> MENKTETTVRRRRRIILFPVPFQGAINPILQLANVLYSKGFSITIFHTNFNKPKTSNYPHFTFRFILDNDPQDERISNLPTHGPLAGMRIPIINEHGADELRRELELLMLASEEDEEVSCLITDALWYFAQSVADSLNLRRLVLMTSSLFNFHAHVSLPQFDELGYLDPDDKTRLEEQASGFPMLKVKDIKSAYSNWQILKEILGKMIKQTKASSGVIWNSFKELEESELETVIREIPAPSFLIPLPKHLTASSSSLLDHDRTVFQWLDQQPPSSVLYVSFGSTSEVDEKDFLEIARGLVDSKQSFLWVVRPGFVKGSTWVEPLPDGFLGERGRIVKWVPQQEVLAHGAIGAFWTHSGWNSTLESVCEGVPMIFSDFGLDQPLNARYMSDVLKVGVYLENGWERGEIANAIRRVMVDEEGEYIRQNARVLKQKADVSLMKGGSSYESLESLVSYISSLLEHHHHHH

UGT76G1 is a UDP-glucose (UDPG)-dependent glycosyltransferase, where UDPG is the sugar donor and UDP is released after sugar transfer. UGT76G1 alone performs β (1–3) glycosylation of Reb D and Reb M in S. rebaudiana. Our data establish that UGT76G1 can transfer glucose in a β (1–3) manner to an existing glucose A at both the R1 and R2 positions (“ends”) of the steviol aglycone. The enzyme UGT76G1 shows an unusual degree of plasticity in substrate recognition; it is able to transfer a glucose to two different ends of some steviol glycosides despite having a single active site.

We have determined the structures of complexes of both the wild type and H25A mutant of UGT76G1 with UDP, the wild type with UDP and Reb A, and the wild type with UDP and Rubu. We propose that His 25 is the general base, which deprotonates the 3-hydroxyl of the accepting glucose A to activate it as a nucleophile. Asp 124 forms a dyad with His 25, suggesting it could play an important catalytic role in relaying protons off and on His 25. The H25N mutation completely eliminates the activity on both R1 and R2 sites as judged by MS. A trace of the product can be detected by MS in the R1 reaction of H25A, the kcat value of such a reaction is 10–5 of that of the wild-type value in the steady-state enzyme assays. The inactivity of the His 25 mutation indicates that the same catalytic machinery is responsible for the sugar transfer at both the R1 and R2 ends. The structure of H25A shows that a cluster of ordered water molecules occupy the position of His 25 and form hydrogen bonds to Asp 124, which might act as a much worse proton relay for the trace activity. The H25N mutation prevents a similar water molecule arrangement.> AHHHHHHGSNKRFPFPVGEPDFIQGDEAIARAAILAGCRFYAGYPITPASEIFEAMALYMPLVDGVVIQMEDEIASIAAAIGASWAGAKAMTATSGPGFSLMQENIGYAVMTETPVVIVDVQRSGPSTGQPTLPAQGDIMQAIWGTHGDHSLIVLSPSTVQEAFDFTIRAFNLSEKYRTPVILLTDAEVGHMRERVYIPNPDEIEIINRKLPRNEEEAKLPFGDPHGDGVPPMPIFGKGYRTYVTGLTHDEKGRPRTVDREVHERLIKRIVEKIEKNKKDIFTYETYELEDAEIGVVATGIVARSALRAVKMLREEGIKAGLLKIETIWPFDFELIERIAERVDKLYVPEMNLGQLYHLIKEGANG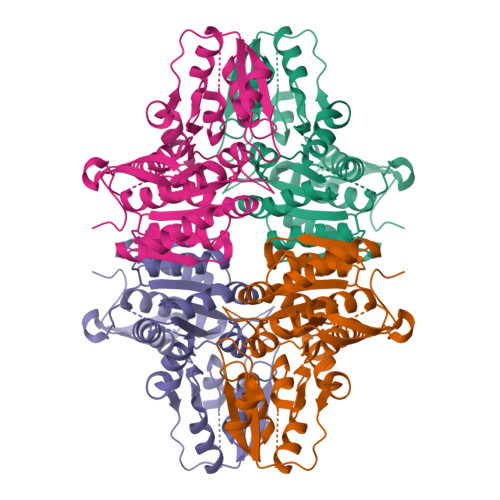KAEVKLISKIGGEVHTPMEIFEFIRREFK The T4 replication system centers on a holoenzyme complex that is assembled from the DNA polymerase (gp43) and the sliding clamp (gp45) loaded onto a primer/template junction by the clamp loader complex (gp44/62) in the presence of ATP. The sliding clamp plays a crucial role by encircling the DNA double helix and anchoring the polymerase to the template. Sequence analysis reveals that T4 polymerase contains three main structural regions: an N-terminal domain, a 3′-5′ exonuclease domain responsible for proofreading activity, and a C-terminal polymerase domain. The T4 gp45 sliding clamp forms a trimeric ring structure, with each of the three monomers composed of structurally similar N-terminal and C-terminal domains (NTD and CTD).

Three-dimensional classification of these two-polymerase complex particles yielded three distinct 3D EM maps, designated as states 1, 2, and 3, with overall resolutions of 3.57 Å, 3.7 Å, and 3.74 Å, respectively. Notably, particle distribution shows nearly equivalent populations with bound DNA entering the right polymerase (state 1; 54%) compared to those with DNA entering the left polymerase (states 2 and 3 combined; 46%). In both states 1 and 2, the DNA substrate remains displaced from the polymerization active site in either polymerase, with the primer 3′ terminus positioned 16 Å away from the catalytic residue Asp-620 and the finger domain maintaining an open conformation. In state 1, the left polymerase thumb is elevated 10 Å higher than its right counterpart while the left polymerase thumb residues Lys-797 and Phe-796 bind the duplex DNA. Concurrently, the right polymerase thumb establishes DNA contacts through residues Asn-783, Asp-784, Lys-787, Tyr-788, Lys-797, and Phe-800, which engage the DNA minor groove, while Arg-704 contacts the DNA backbone. The primer 3′-terminus remains excluded from both polymerization and exonuclease active sites of the right polymerase. As the polymerase exchange progresses from state 2 to state 1, the duplex DNA tilts by 25° toward the right polymerase allowing the P/T junction to approach the polymerization active site of the right polymerase. The sliding clamp adjusts its position to accommodate this DNA movement, and this repositioning causes the original left polymerase to dissociate from the clamp.

>MKEFYISIETVGNNIVERYIDENGKERTREVEYLPTMFRHCKEESKYKDIYGKNCAPQKFPSMKDARDWMKRMEDIGLEALGMNDFKLAYISDTYGSEIVYDRKFVRVANCDIEVTGDKFPDPMKAEYEIDAITHYDSIDDRFYVFDLLNSMYGSVSKWDAKLAAKLDCEGGDEVPQEILDRVIYMPFDNERDMLMEYINLWEQKRPAIFTGWNIEGFAVPYIMNRVKMILGERSMKRFSPIGRVKSKLIQNMYGSKEIYSIDGVSILDYLDLYKKFAFTNLPSFSLESVAQHETKKGKLPYDGPINKLRETNHQRYISYNIIDVESVQAIDKIRGFIDLVLSMSYYAKMPFSGVMSPIKTWDAIIFNSLKGEHKVIPQQGSHVKQSFPGAFVFEPKPIARRYIMSFDLTSLYPSIIRQVNISPETIRGQFKVHPIHEYIAGTAPKPSDEYSCSPNGWMYDKHQEGIIPKEIAKVFFQRKDWKKKMFAEEMNAEAIKKIIMKGAGSCSTKPEVERYVKFSDDFLNELSNYTESVLNSLIEECEKAATLANTNQLNRKILINSLYGALGNIHFRYYDLRNATAITIFGQVGIQWIARKINEYLNKVCGTNDEDFIAAGDTDSVYVCVDKVIEKVGLDRFKEQNDLVEFMNQFGKKKMEPMIDVAYRELCDYMNNREHLMHMDREAISCPPLGSKGVGGFWKAKKRYALNVYDMEDKRFAEPHLKIMGMETQQSSTPKAVQEALEESIRRILQEGEESVQEYYKNFEKEYRQLDYKVIAEVKTANDIAKYDDKGWPGFKCPFHIRGVLTYRRAVSGLGVAPILDGNKVMVLPLREGNPFGDKCIAWPSGTELPKEIRSDVLSWIDHSTLFQKSFVKPLAGMCESAGMDYEEKASLDFLFG[2x];>[3x]MKLSKDTTALLKNFATINSGIMLKSGQFIMTRAVNGTTYAEANISDVIDFDVAIYDLNGFLGILSLVNDDAEISQSEDGNIKIADARSTIFWPAADPSTVVAPNKPIPFPVASAVTEIKAEDLQQLLRVSRGLQIDTIAITVKEGKIVINGFNKVEDSALTRVKYSLTLGDYDGENTFNFIINMANMKMQPGNYKLLLWAKGKQGAAKFEGEHANYVVALEADSTHDF> MNLLNAAPTPYVWKYNPVTGKC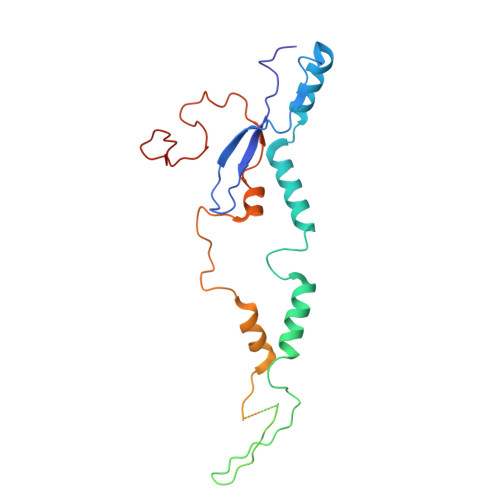AGAQQNYGATIDWVLPGGNSFAYAADEIRRRFPEPAVTRAITARFEAESDQQPYAGPHETNIITADVVRSGPPPSAVYPFDPSGVQRVQLSGGMMGGRTEGRMQLSGGLTEGRMQLAGGAAGKLPTRARPTLRPPRWCGTTLTGNGLPADYPEMTPDAFKYYLRVQGPSQEVDEPGVMSQRQFMTTFLPAMVPHPFDSESPDAFPAYFSSVYKGTNAFEPVFWQG>[4x]MLLHLIYGPTCSGKTDMAIQIAQETGWPVVALDRVQCCPQIATGSGRPLESELQSTRRIYLDSRPLTEGILDAESAHR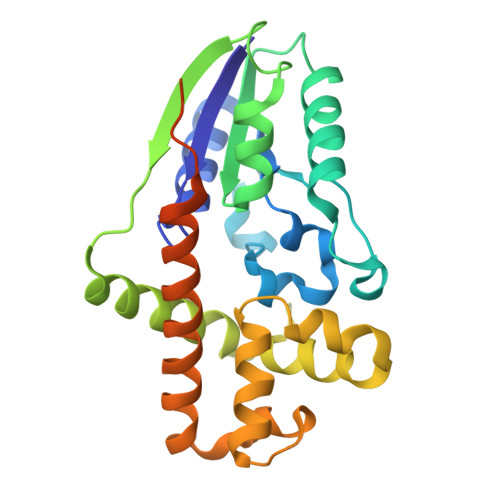RLIFEVDWRKSEEGLILEGGSISLLNCMAKSPFWRSGFQWHVKRLRLGDSDAFLTRAKQRVAEMFAIREDRPSLLEELAELWNYPAARPILEDIDGYRCAIRFARKHDLAISQLPNIDAGRHVELIEAIANEYLEHALSQERDFPQWPEDGAGQPVCPVTLTRIRGSRSHHHHHH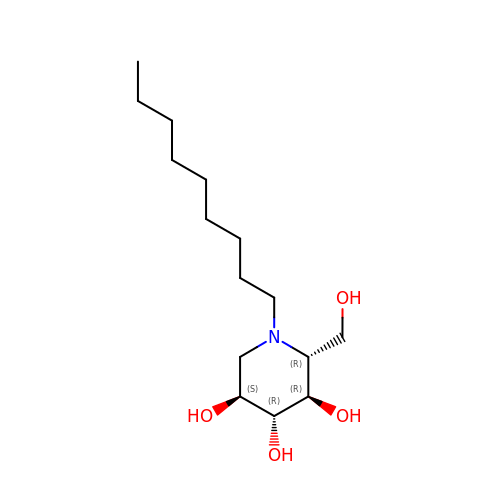(2R,3R,4R,5S)-2-(HYDROXYMETHYL)-1-NONYLPIPERIDINE-3,4,5-TRIOL | C15 H31 N O4 | FTSCEGKYKXESFF-LXTVHRRPSA-N5'-O-(N-ETHYL-SULFAMOYL)ADENOSINE | C12 H18 N6 O6 S | 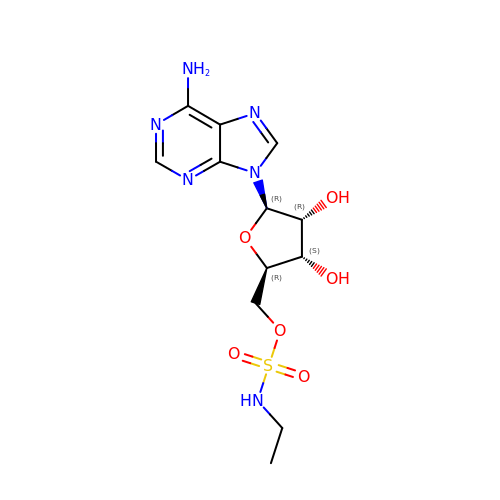ONCSLXAPOGUODU-WOUKDFQISA-N>[2x]MAEQLVEAPAYARTLDRAVEYLLSCQKDEGYWWGPLLSNVTMEAEYVLLCHILDRVDRDRMEKIRRYLLHEQREDGTWALYPGGPPDLDTTIEAYVALKYIGMSRDEEPMQKALRFIQSQGGIESSRVFTRMWLALVGEYPWEKVPMVPPEIMFLGKRMPLNIYEFGSWARATVVALSIVMSRQPVFPLPERARVPELYETDVPPRRRGAKGGGGWIFDALDRALHGYQKLSVHPFRRAAEIRALDWLLERQAGDGSWGGIQPPWFYALIALKILDMTQHPAFIKGWEGLELYGVELDYGGWMFQASISPVWDTGLAVLALRAAGLPADHDRLVKAGEWLLDRQITVPGDWAVK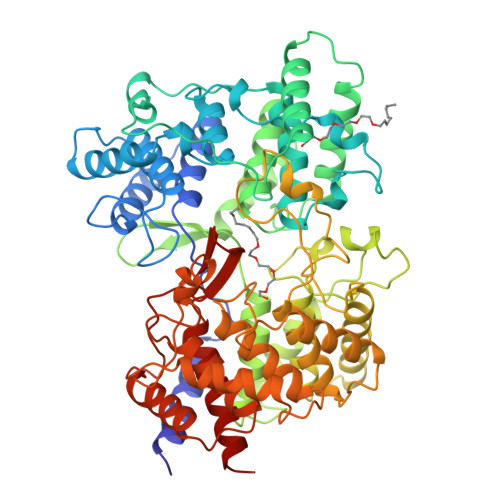RPNLKPGGFAFQFDNVYYPDVCDTAVVVWALNTLRLPDERRRRDAMTKGFRWIVGMQSSNGGWGAYDVDNTSDLPNHIPFSDFGEVTDPPSEDVTAHVLECFGSFGYDDAWKVIRRAVEYLKREQKPDGSWFGRWGVNYLYGTGAVVSALKAVGIDTREPYIQKALDWVEQHQNPDGGWGEDCRSYEDPAYAGKGASTPSQTAWALMALIAGGRAESEAARRGVQYLVETQRPDGGWDEPYYTGTGFPGDFYLGYTMYRHVFPTLALGRYKQAIERR> RQAKKQTKLAAKNARKMKESKGLLLEGKKTALCMNL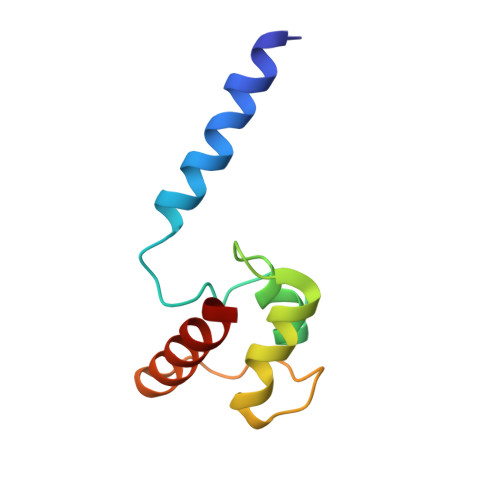MQNTGIAWYRSLQVCKHLEMHRRAPVPRVTAGFREKVTQAVAVVKLG>[2x]SGSTQACLPVGSRKNGMNVNFYKYSLQDSTTY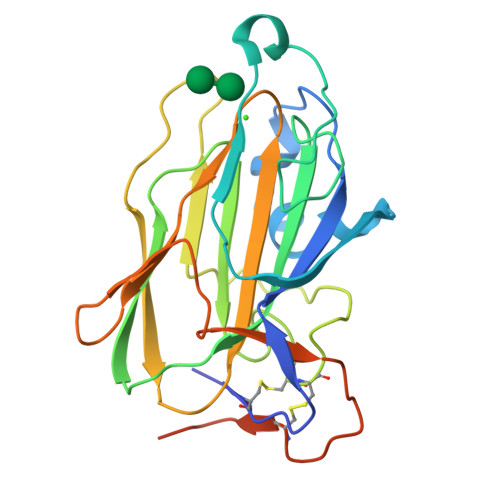SDPQYMAYKYSDTKKLGSVSGQTHLSIYYDLNTAFWNTASWSSDLFGFYTTPTNVTVEMTGYFLPPQTGSYTFKFATVDDSAILSVGGSIAFECCAQEQPPITSTDFTINGIKPWGAAAPTDIKGSTYMYAGYYYPIKIVYSNAKALARLPVSVVLPDGTEVNDDFEGYVYSFDDDLSQSNCTIPDPSKHTTSLEVLFQGPHHHHHH>[2x]DPDVAELFFKDDPEKLFSDLREIGHGSFGAVYFARDVRNSEVVAIKKMSYSGKQSNEKWQDIIKEVRFLQKLRHPNTIQYRGCYLREHTAWLVM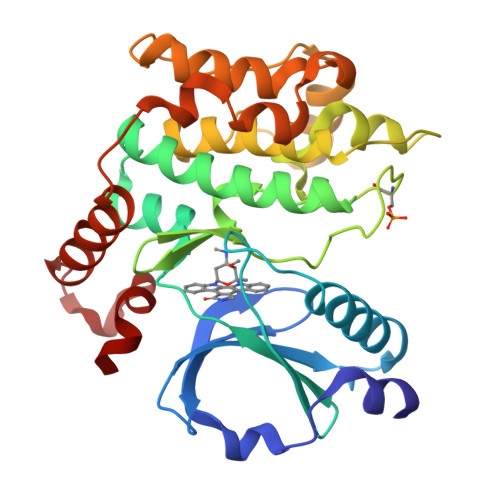EYCLGSASDLLEVHKKPLQEVEIAAVTHGALQGLAYLHSHNMIHRDVKAGNILLSEPGLVKLGDFGSASIMAPANSFVGTPYWMAPEVILAMDEGQYDGKVDVWSLGITCIELAERKPPLFNMNAMSALYHIAQNESPALQSGHWSEYFRNFVDSCLQKIPQDRPTSEVLLKHRFVLRERPPTVIMDLIQRTKDAVRELDNLQYRKMKKILFQEA butane-2,3-dione | C4 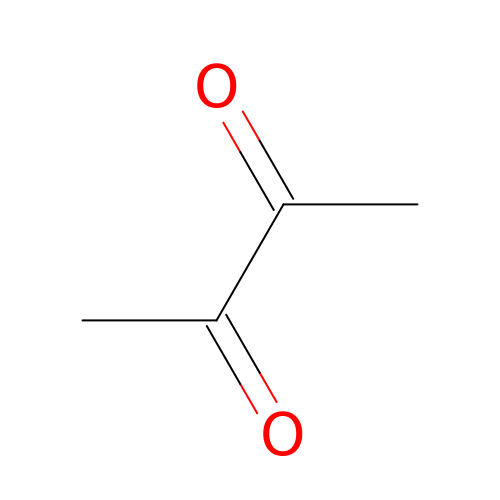H6 O2 | QSJXEFYPDANLFS-UHFFFAOYSA-N> GSHMPKRVALGCDHAAY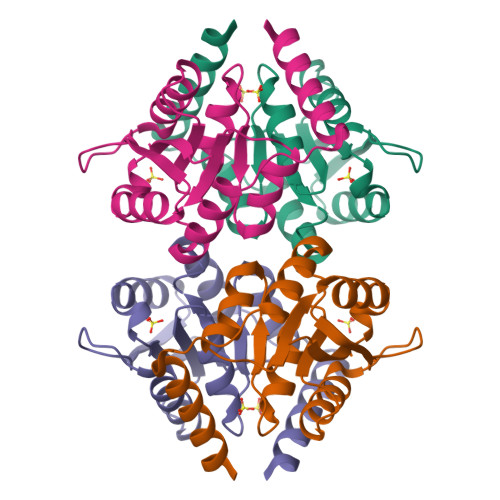ATHQEIMDMVNASGAASKVMYMGPSSDTSVDYPDYAAQVCEAILKGEADTGILVCGTGIGMSIAANKFRGIRAALCYDHVTAQLSRQHNNAHILCIGVRTSGMEVIRDIIETFLTTEPLAEGRHGNRVDKITVIEEEQMKDEQRWCFSGCGGLKEEGK> GAGCA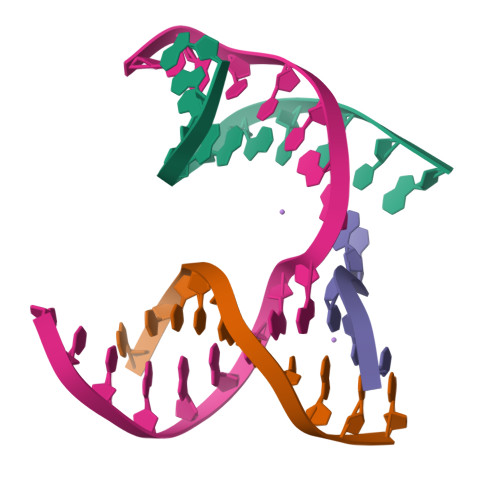GACCTG;> ACACCACTCA;> CATGT;> TCTGAGTGGGGTCTGC> MERVNVVGAGLAGSEAAWTLLRLGVPVRLFEMRPKRMTPAHGTDRFAEIVCSNSLGGEGETNAKGLLQAEMRRAGSLVMEAADLARVPAGGALAVDREEFSGYITERLTGHPLLEVVREEVREIPPGITVLATGPLTSEALAEALKRRFGDHFLAYYDAASPIVLYESIDLTKCFRAGRYGQSADYLNCPMTEEEY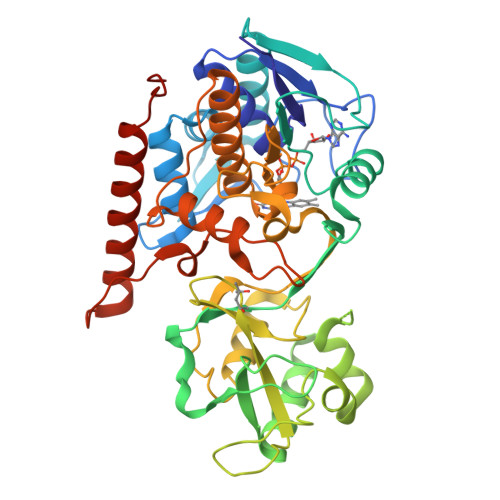RRFHQALLEAQRHTPHDWEKLEFFEACVPVEELARRGYQTLLFGPMKPVGLVDPRTGKEPFAVVQLRQEDKAGRMWSLVGFQTGLKWPEQKRLIQMIPGLENAEIVRYGVMHRNTYLNAPRLLGETLEFREAEGLYAAGVLAGVEGYLESAATGFLAGLNAARKALGLPPVAPPEESMLGGLVRYLATANPEGFQPMYANWGLVPPVEGRMGKKEKRQAMYRRGLEAFSAWLSGLNPPLPRPEAALV>MNMVMLTIDGKQVQVEKGTTIKKAAEKLGIEIPGLCDDNDLKPFGACRLCVVEDARGNLVASCHTPVREGMVVKTNSPKVLKARRVILELLLSSHNADCFECDKNLHCKLQKYAYELNIRNIRFKGEKRNYEIKDNGPIYYDPNKCILCGKCVRICEEVQHICAIDFASRGFKAYISTPFEKPLLESDCIFCGQCVRVCPTGALAEKTDIERIYEAISDPNKVVVVQVAPAVRVALGEEFGLEPGEIVTGKMVAALKRLGFDKVFDTQFAADMTIVEETAELVERLEKGENFPMFTSCCPSWILAVEKFYPELIPNISTARSPQQIFGAIAKNYYAKKIGVARENMFVVSVMPCIGKKFEATRPEFNNDVDAVLTTRELARMIKESGIDFIKLEEENFDSPLGESTGAAAIFGVTGGVMEAALRTAYSIMTGEELEGDKIEFTAVRGLEGIKEAEVDIKGKKVRIAIANGIGNAKKLIEKIKSGETKYDFVEVMACPGGCMSGGGQPYTDDPEFRKKRMEGIYKNDRNLPKRKSHENEEVKKVYEEYYEKPCGPKAHEELHTHYHSRKKEY[2x];>MVKLKSIQELENLREKIKEAKKKEKIVIRICGGTGCRASGSLAVRDELVKVLKREGFANVDVNLSSDCLENTSEVHVKMTGCQGFCAQGPLMTIEPLGVFYVGVKPEDVEEIVEKSIKKNEIIERLLYHDPATGKTYVKRDENPFYAKQTRLVLKHCGTVDPASVYDYIAEGGYSAIAKALTMDRKQIIDEVIKSGLRGRGGAGFPTGEKWLGAYKNQSPKKYIICNGDEGDPGAFMDRSVMEGDPHKVIEGMMIGAYAIGSDEGYIYVRAEYPLAVQMLRKAIEECEKLGLLGDNILGTGFSFRLHVREGAGAFVCGESTALTYSIEGKRGMPRVRPPRTNECGLWEMPTVLNNVETFACIPEIILNGGEWFASIGT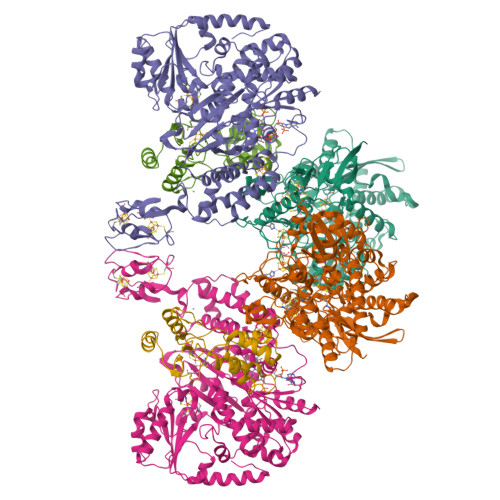PTSTGTKIFALSGKVNRTGLVEVPMGLKLRELIFDIGGGIANNKKFKAVQLGGPSGGCVPESQLDLPIDFDSLSKAGAIMGSGGVVVVDEDTCMVDFAKFFTNFIVEESCGKCIPCREGNKKMLEILERITEGKGKEGDIELLEELGDVIISASLCGLGKTAPNPVLSTIKHFRDEYEAHIRDKKCPAGACQALAAYKIDPGKCIGCGKCVKVCPVGAISGEKKKPHVIDQSKCIKCGACAENCPKGAIYKG[2x];>[2x]MCNCCCKGSKDPRFEKVDEILSKLANERGALIAILQHVQHEFGYLPEDVIFYIASKTGIPASKIYGVATFYAQFHLKPRGKYVIRVCLGTACHVKGANKILAEFEKQLGIKAGETTSDLKFTLERVGCLGACGLAPTVMVNEKTYGKMTPEKVSEVLKEYSDVEAAASAQ(1~{R},2~{S})-2-[(2,4-dimethylpyrimidin-5-yl)oxymethyl]-~{N}-(5-fluoranylpyridin-2-yl)-2-(3-fluorophenyl)cyclopropane-1-carboxamide 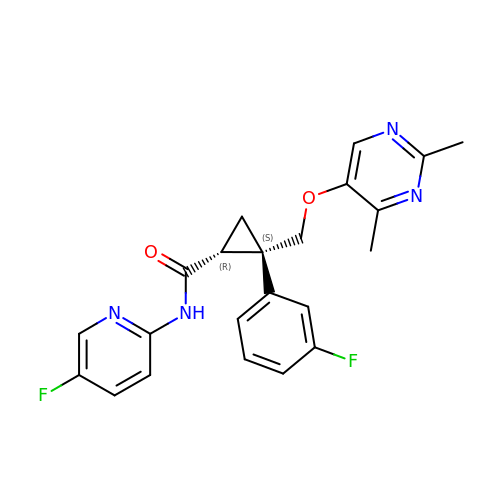| C22 H20 F2 N4 O2 | MUGXRYIUWFITCP-PGRDOPGGSA-N>[2x]GQRWELALGRFWDYLRWVQTLSEQVQEELLSSQVTQELRALMDETMKELKAYKSELEEQLTPVAEETRARLSKELQAAQARLGADMEDVRGRLVQYRGEVQAMLGQSTEELRVRLASHLRKLRKRLLRDADDLQKRLAVY;>[2x]PFPKPTLWAEPGSVISWGSPVTIWCQGSLEAQEYRLDKEGSPEPLDRNNPLEPKNKARFSIPSMTEHHAGRYRCHYYSSAGWSEPSDPLELVMTGFYNKPTLSALPSPVVASGGNMTLRCGSQKGYHHF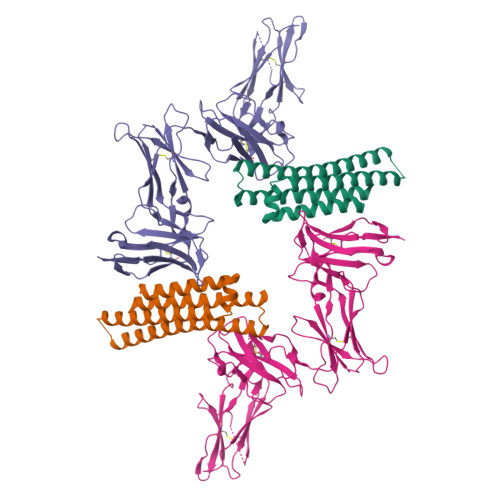VLMKEGEHQLPRTLDSQQLHSGGFQALFPVGPVNPSHRWRFTCYYYYMNTPQVWSHPSDPLEILPSGVSRKPSLLTLQGPVLAPGQSLTLQCGSDVGYDRFVLYKEGERDFLQRPGQQPQAGLSQANFTLGPVSRSHGGQYRCYGAHNLSSEWSAPSDPLNILMAGQIYDTVSLSAQPGPTVASGENVTLLCQSWWQFDTFLLTKEGAAHPPLRLRSMYGAHKYQAEFPMSPVTSAHAGTYRCYGSYSSNPHLLSFPSEPLELMVSG>[4x]DRHHHHHHKLDRKPRHYEINLDEPPSQRWNQVIKDHLEYLPGVVEETKKYIPKPLQPFVWWAASKIDRYFTTEIQEELKGIASESGLPIGEIVGMNILYDVAAFDRRHIFGLG;>[4x]CTSIVAQNSAGQIIHGRNLDYDMTELLKNITIHVDFVRNGTIQYSGLTFALYNGVLTGQRPGEYSVS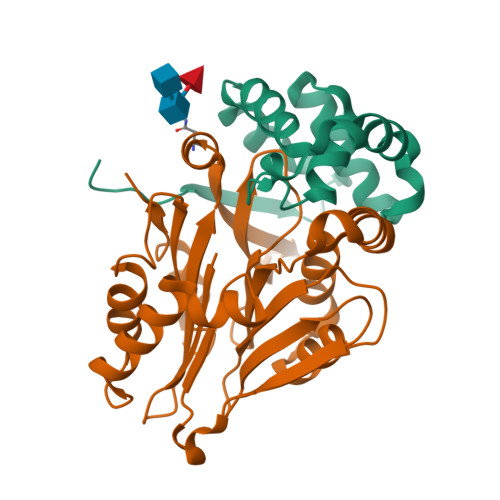LNARYSGAYIDNILMEFYTKFKRPVSFFIRDVLENQATYTEAVDAFSRTHLFSPSYIIVAGIKKNEGVVISRNRWSAANVYPLNVDANQWFLVETNFDNWKKQGDDRRITAIQKLKELGRRNFDEKSMVEVLSTVPVRNNLTVFSTVMVPGLPDSADYFRQSTWILP>[2x]GAMDTRKNVSGAERKIWSLIRDCSGKLEGVTETSVLEVLLIVSRVLGIRKE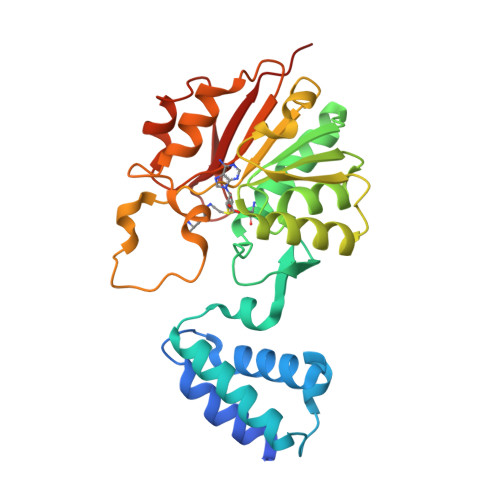DLFLKDLGVSPTEEKRILELVEKRASGYPLHYILGEKEFMGLSFLVEEGVFVPRPETEELVELALELIRKYGIKTVADIGTGSGAIGVSVAKFSDAIVFATDVSSKAVEIARKNAERHGVSDRFFVRKGEFLEPFKEKFASIEMILSNPPYVKSSAHLPKDVLFEPPEALFGGEDGLDFYREFFGRYDTSGKIVLMEIGEDQVEELKKIVSDTVFLKDSAGKYRFLLLNRRSS>GMADLTHEFWDRLEDVRSGMLGIKGQGRLIPMSPQTDDDAPGAIWFITAKGTDLAKGVAAGPQPAQFVVSDDGEGLYADLDGTLERSTDREALDEFWSFVADAWFDGGQHDPDVCLLKFTPASGEISITEGGGARF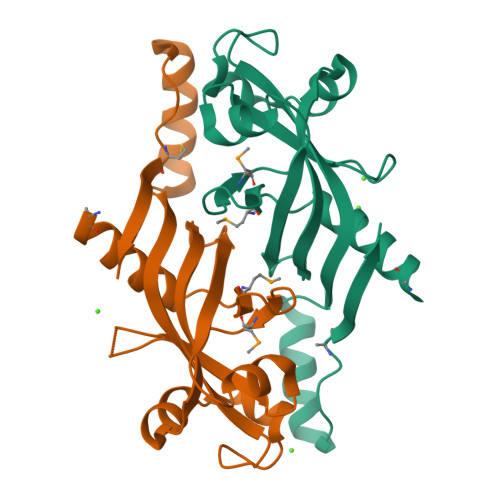LYEIAKAHLTDETPDMGEQATVTF[3x]>[2x]EAEEDGDLQCLCVKTTSQVRPR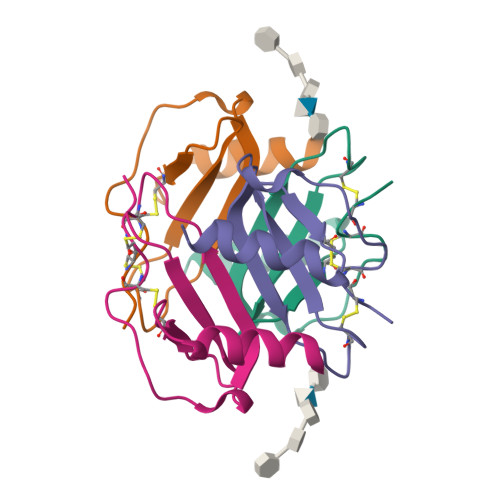HITSLEVIKAGPHCPTAQLIATLKNGRKICLDLQAPLYKKIIKKLLES>GHMDTSKVKVGVMAGAEAQVAEVAAKVAKEKYGLDVELVTFTDYVTPNAALDDGSIDMNAFQHKPYLDRQVEDRDYKLTIA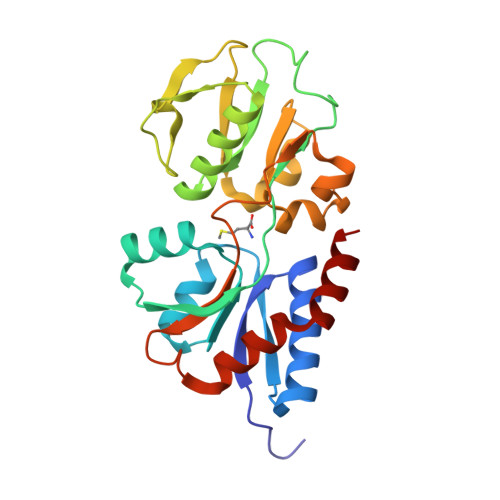GNTFVYPIAGYSKQVKSVAALADGVRIAVPNDPTNLGRSLLLLEQQGLIKLRPEVGLLATVRDIVENPKNITIMELDAAQLPRSLDDVALSIINTTYASSINLTPEKDGVFVEDKESPYVNLIVARQDNVQNENVQNFVKAYQTEEVYTAAKEIFK[2x]3-[(4,6-dipyridin-3-yl-1,3,5-triazin-2-yl)amino]-4-methyl-~{N}-[3-(trifluoromethyl)phenyl]benzamide 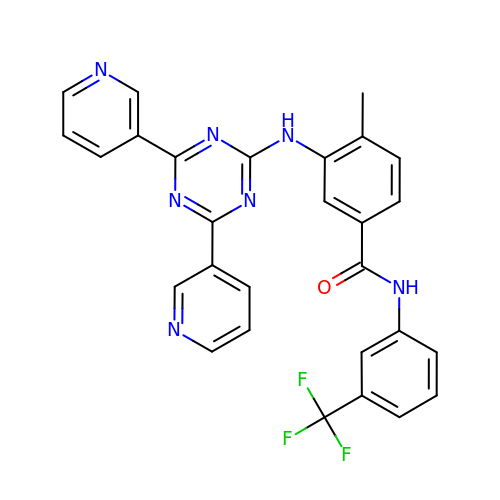| C28 H20 F3 N7 O | FQDJXKXBKFLPSH-UHFFFAOYSA-N> MGHHHHHHEFMSKTDYILRALSKISHKRWEHYIINRVVHTLDDPDIEFVCQQCIRKEGHLGKIYLADLLFPQLNLYLEIDEAHHDSNDARKADAVRRLDIVEATGFQEERIPASNITLSEVNKLVDEFVRLVKDKKEELENQGLFFRWDYDERYSAKKHINTGYMAVGPNSVFRYHRDALQCFGYRREGHHQSGGWALPAEVAQSIGLTGRVMVWFPRLYEAGEWKNALSADGNKITEQSLNATRNYQETWDYRIVMAHSRDELNRTLYRFLGVFAIDVDKSSDEVKVFSRVYSRVNVYRSQN

The endonuclease PvuRts1I from Proteus vulgaris (strain) has been reported to be a dimer like most endonucleases that catalyze double strand breaks. PvuRts1I makes a double strand break approximately in the middle between the two sites (the precise pattern is 5′-CN11–13↓N9–10G-3′, where the arrow denotes the cleavage site and C the modified base). Here, we report the crystal structure of PvuRts1I at 2.35 Å resolution. The structure reveals an N-terminal PD-(D/E)XK domain in agreement with an earlier prediction and a previously unrecognized C-terminal SRA domain.

Crystals belonged to space group P4(1)2(1)2, contained one molecule of PvuRts1I in the asymmetric unit and diffracted up to 2.35 Å resolution. The crystal structure reveals that PvuRts1I is a two-domain protein. We therefore conclude that the N-terminal part of the enzyme (residues 1–140) harbors the nuclease activity and henceforth refer to it as the catalytic domain. Therefore, the C-terminal domain of PvuRts1I (residues 141–293) will be referred to as its SRA domain in the following. The canonical ‘(D/E)XK’ motif in PvuRts1I is changed to ‘EID’, with Glu68 in the role of the acidic residue of the motif and an aspartate in the place of the expected lysine residue. Metal ions are not present in the active site because crystals were grown in the absence of divalent metal ions. The pocket is formed mainly by Pro207, Trp205, Trp215, Asn217 and Glu228. Interestingly, we see an isolated large peak of electron density close to the expected location of the glucosylhydroxymethyl group in the pocket for the flipped base. In agreement with the biochemical data for the PvuRts1I variant used in this work, we do not find the predicted dimer in the crystal. Thus, it appears that the tag, despite not being located in the dimerization interface, together with crystallization forces could be responsible for the unusual monomeric state of the protein in the crystal.> WV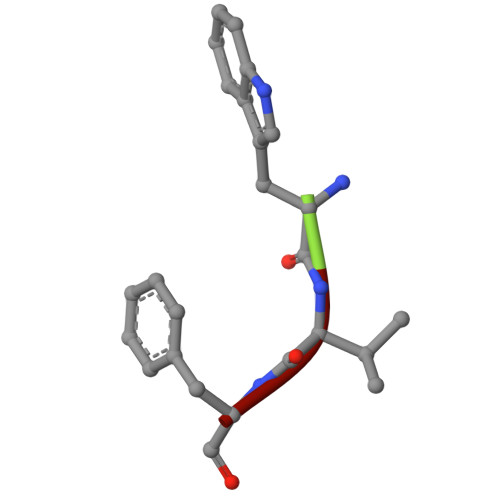F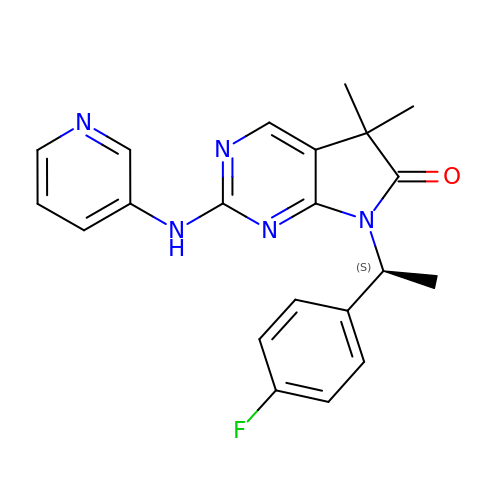7-[(1~{S})-1-(4-fluorophenyl)ethyl]-5,5-dimethyl-2-(pyridin-3-ylamino)pyrrolo[2,3-d]pyrimidin-6-one | C21 H20 F N5 O | KWJOTUQSCIOUKF-ZDUSSCGKSA-N>MGHHHHHHGRAMNNPAIKRIGNHITKSPEDKREYRGLELANGIKVLLISDPTTDKSSAALDVHIGSLSDPPNIAGLSHFLQHMLFLGTKKYPKENEYSQFLSEHAGSSNAFTSGEHTNYYFDVSHEHLEGALDRFAQFFLSPLFDESAKDREVNAVDSEHEKNVMNDAWRLFQLEKATGNPKHPFSKFGTGNKYTLETRPNQEGIDVRQELLKFHSAYYSSNLMAVVVLGRESLDDLTNLVVKLFSEVENKNVPLPEFPEHPFQEEHLKQLYKIVPIKDIRNLYVTFPIPDLQKYYKSNPGHYLGHLIGHEGPGSLLSELKSKGWVNTLVGGQKEGARGFMFFIINVDLTEEGLLHVEDIILHMFQYIQKLRAEGPQEWVFQELKDLNAVAFRFKDKERPRGYTSKIAGILHYYPLEEVLTAEYLLEEFRPDLIEMVLDKLRPENVRVAIVSKSFEGKTDRTEEWYGTQYKQEAIPDEVIKKWQNADLNGKFKLPTKNEFIPTNFEILPLEKEATPYPALIKDTAMSKLWFKQDDKFFLPKANLNFEFFSPFAYVDPLHSNMAYLYLELLKDSLNEYAYAAELAGLSYDLQNTIYGMYLSVKGYNDKQPILLKKIIEKMA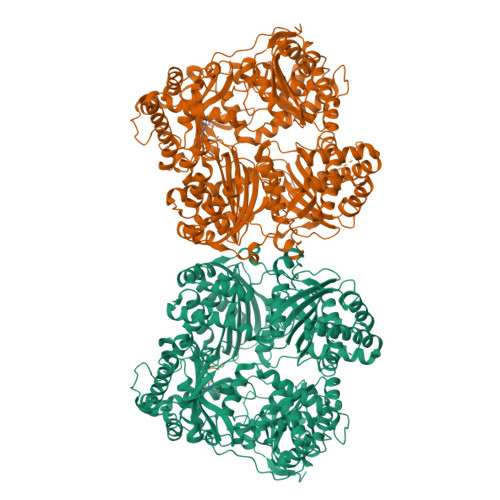TFEIDEKRFEIIKEAYMRSLNNFRAEQPHQHAMYYLRLLMTEVAWTKDELKEALDDVTLPRLKAFIPQLLSRLHIEALLHGNITKQAALGIMQMVEDTLIEHAHTKPLLPSQLVRYREVQLPDRGWFVYQQRNEVHNNSGIEIYYQTDMQSTSENMFLELFAQIISEPAFNTLRTKEQLGYIVFSGPRRANGIQGLRFIIQSEKPPHYLESRVEAFLITMEKSIEDMTEEAFQKHIQALAIRRLDKPKKLSAESAKYWGEIISQQYNFDRDNTEVAYLKTLTKEDIIKFYKEMLAVDAPRRHKVSVHVLAREMDSNPVVGEFPAQNDINLSQAPALPQPEVIQNMTEFKRGLPLFPLVKPHINFMAAKL[2x]> GUGCGACAAGAAGUUCAGGAAGGGAUUGAGGUGAAAGUCCUCCUCCCGAAUCGUUCAUGGGAGAGUCUAUCCAGACUUGCGUAGCGAGUAAUCGCUAGGUGAGAAGCUCUGGAGACAAUGUACCU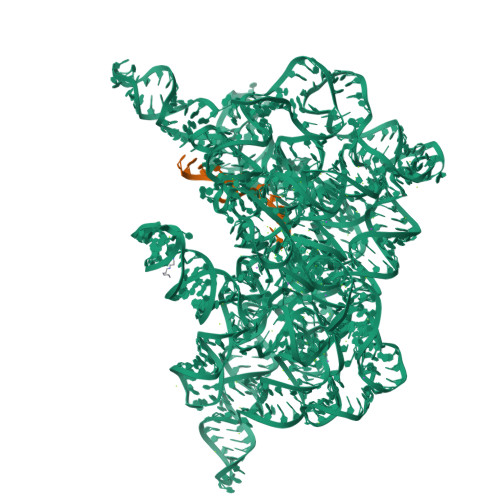GCCCUUCAAUUGGAGGUGCCAGGGCUAGGCUUUGUUCCUAUGGCUAGCGAAAGCGAAUACAGGUUAUUAGGCGUCGUGAAAACAAAACUCUUUCGACAUAAGGGAGAGGCUCGUAGAUGAGUUACCCUCCUUUUUAUGGGGUAACUGAACGAUCAAUAUCUACCGGCGUAGACUGUGAGCCUAAAGGAAACGAAUGAAAGUGUCCCUUCCUGGGAACUUGGUAAGCCCAAUAGACUCCCUCUGGGAAACCAGAGGAGGAGUAAGAGCAAUCUUACUUAUCGUCUAGUGGGUAAAAGACAUAAUAGGAAGCAAAUGCUUGGUUGUAACGAUCGAGAUAGAAUCUGUUGAUUUAAGCUGAAAGGCUGCAGACUUAUUAAAUGGGUGUUCUGCUGUAUGGCGUUCGCGCCUAAGCAGCAGAAUGCGUGAGCCGUGUGCGAUGAAAGUCGCAAGCACGGUUCUGAUGGGGGGAAAACGAGAGAUCGUCUACCUAUCCAACUCAA;> UGUUUAUUAAAAA> SKQFTSSTSYNRG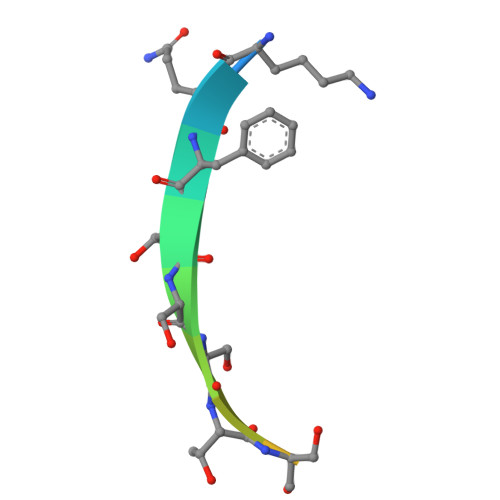DS Here, we present a computational protein design strategy to repurpose drug-inhibited protein-protein interactions as OFF- and ON-switches. The designed binders and drug-receptors form chemically-disruptable heterodimers (CDH) which dissociate in the presence of small molecules. Therefore, we devised a strategy to design chemically-controlled switches by repurposing protein components and small molecules involved in the inhibition of protein-protein interactions (PPI). Previously, we reported the design of chemically disruptable heterodimers (CDH) from known protein: peptide-motif complexes, by transferring the peptide motif from the disordered binding partner to globular proteins and using the known PPI inhibitor as a chemical disruptor.

To further expand the panel of CDHs and the chemical space of small-molecule disruptors, we designed a novel CDH-3, based on the starting point of the interaction between p53 and mdm2. Particularly, the dihydroisoquinoline derivative, NVP-CGM097 (Drug-3), is currently undergoing phase 1 clinical trials. We performed a structural search over approximately 11,000 putative protein scaffolds and after the design stage we selected for experimental characterization three designs which we refer to as LD4, LD5 and LD6. From these three designs, LD6 a design based on a thioredoxin protein from mouse, showed the best biochemical behavior being monomeric in solution and a melting temperature of 62 ˚C. LD6 bound to mdm2 with a Kd of 4 nM as determined by SPR, showing a higher binding affinity than those reported for the wild-type p5317-29 peptide (820±60 nM) or the stapled p53 peptide which we used as the input peptide motif (12±3 nM). Next, we tested if Drug-3 promoted the dissociation of the mdm2:LD6 complex by SPR and determined an IC50 of 106 nM. These results were also confirmed using SEC-MALS where the drug dissociated the complex into two monomers. To evaluate the structural accuracy of the designed CDH-3, we solved the crystal structure of the mdm2:LD6 complex at 2.9 Å resolution by X-ray crystallography. The structure of the complex closely matched our computational model, with backbone RMSDs of 0.37 Å over the overall structure and 0.24 Å over the p53 motif region. The conformation of key residues observed in the native interface were closely mimicked in the crystal structure of LD6 in complex with mdm2.

> MEFSQIPASEQETLVRPKPLLLKLLKSVGAQKDTYTMKEVLFYLGQYIMTKRLYDEKQQHIVYCSNDLLGDLFGVPSFSVKEHRKIYTMIYRNLVVVNQQESSDSGTSVSENLE;> MATHTAQTQTHLNFTQIKTAFALYWALLEAQGKPVMLDLYADWCVACKEFEKYTFSDPQVQKALADTVLLQANVTANDAQDVALLKHLNVLGLPTILFFDGQGQEHPQARVTGFMDAETFSAHLRDRQPLEHHHHHH> GSISLSQEHIDHLNKTLVELSPQEVLRWAVVTFPNLYQTTAFGLTGLVILDMISKTKPVDLIFIDTLHHFPQTYDLVRKVAAAYQPTLHIYKPKGVESEEEFAKKHGDSLWESNDDLYDFLVKVEPAQRAYKELGVNAVLTGRRKSQGGARAALPVIEVEESSGIIKINPLWNWDFAQV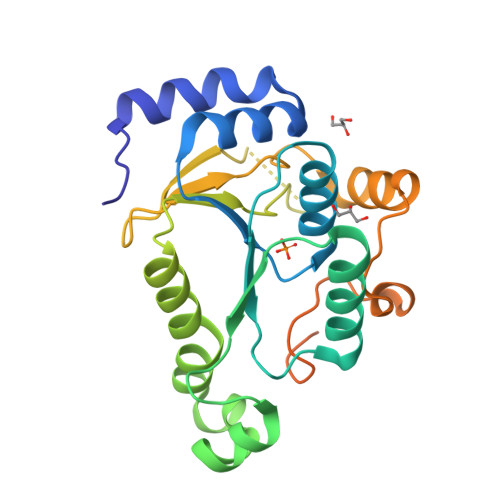KAYITENAVPYNELLDLGYKSIGDWHSTVAVADGEDERSGRWKGKAKTECGIHETSRFAQYLASTSS> K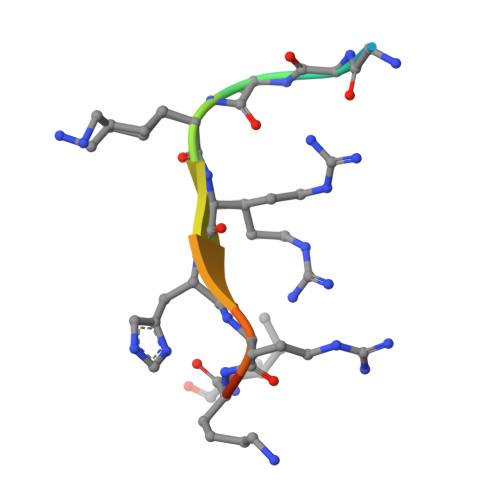GGAKRHRKIL> MDTAHPTASWEQLGERFYRKIQLYTQVFDQDFDLDNYIVTGAPYGGAIALYRDDEKLVAYQPSRSSRPTIDICSLSGKLLRRISWDQGPIKGVGWSEDEKLLIVMVDGTVRCYFDLQSEFTQFSLGHGAEEHGVKSCRFYSHGLVALLGNNALVSVSSYDEPRPKLLASPPEGRVYSWNIIPPAYSLSRSVEVLLSVNQTIYVCDASECEDRFLDIGPFSHIAVSPNGRFCALYTTTGKVHVITSDFQSRLSEHDTKSKIAPNYFEWCGNDAVVIAWDDEVHLVGPSGSLARFFYDSGRIHLIPDFDGVRILANDRCDFLQKVPDVIEEVFGLGADSPASILLDAVEQLEMKSPKADDNIQLIRPHLVEAVDTCVSAAGQEFSIHWQKQLLKAASFGKSVLDIYNSDDFVDMCETLRVLNAVRFYEVGLPLSYEQYQRLSPSGLISRLLNRHEYLLAIRIADHLRLPTDKIHVHWASAKVRLGSEDDDTICRKIVEKLSGKPGISFEVIARTAYEEGRTRLATELLNHEPRAGRQVPLLLSMEEDELALDKAIESGDTDLIYFVIHQLRRKLPLASFFRVVSSRPTASAMVEALARNSDGDGNEDTALLKDLYYQDDRRLDGASVFIREALQQPETRTASDKLDLAANLLQGNQKEHVFELGALKEAKMLLRMQETFERDLTDSFVGLSVNQT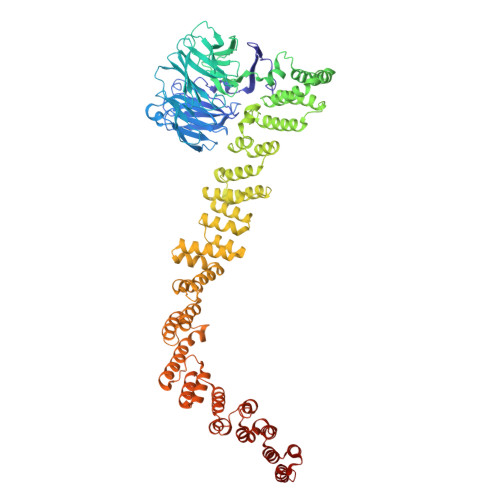MFKLIKLGYHGRAKKIQSEFKVPERVAWWIRLQALVAKRDWNEIEEISRQRKSPIGWEPFFNQVLQAGNPRLAATFIPKCTNLEPGQTITMYEKCGMRVKAAEEAVRLKDTEAWNRLLEAAGRNTAEGREIERLGATVFKK>[4x]QTSCD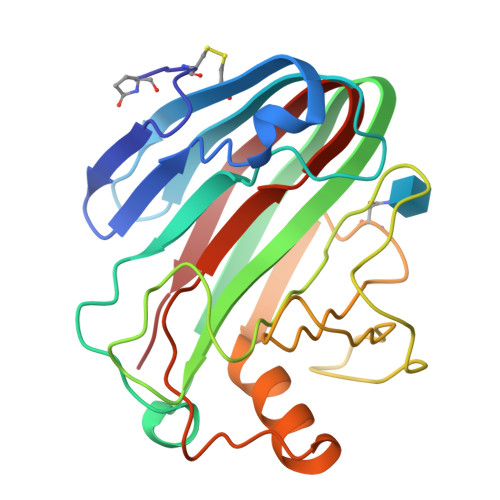QYATFSGNGYIVSNNLWGASAGSGFGCVTSVSLNGAASWHADWQWSGGQNNVKSYQNVQINIPQKRTVNSIGSMPTTASWSYSGSDIRANVAYDLFTAANPNHVTYSGDYELMIWLGKYGDIGPIGSSQGTVNVGGQTWTLYYGYNGAMQVYSFVAQSNTTSYSGDVKNFFNYLRDNKGYNAGGQYVLSYQFGTEPFTGSGTLNVASWTASIN>SNAMEETEAVQQDIEALEREIQTIKIQIANAHSGASKDEVKIPDAYKQFLSENINFSNLMRKDENTTLSINLSPRKPGTTTGQIQGIDSSIRSNFGVSSGHNEVAGFKSITDFVQWENSVRLIGVSLFPVNYDNIEFMGIRLELFDELSLKYDPPFYVILKPSVKRLGIWELFKHNLPKYINIHQHWQLITKDTDTSDSNIMKFANLCYKDLLKVHSRVQFFRKLEGNYVNDKQYSLLHIDNMGLNVSFRLGADIIKIKVDDGDDEIIDCTFNGEKNISLLGSIYGITNRFQSIIM[2x];>MDFTSSSGVLDSERNTGSNDSDEPSSHSDVIETEELKLIKLQEHKNNLLRQRSELLDQLSQTRVVEPRSVQLDDKLLLKLLRRNDNAVSDSSQSSNNPLPRVLPS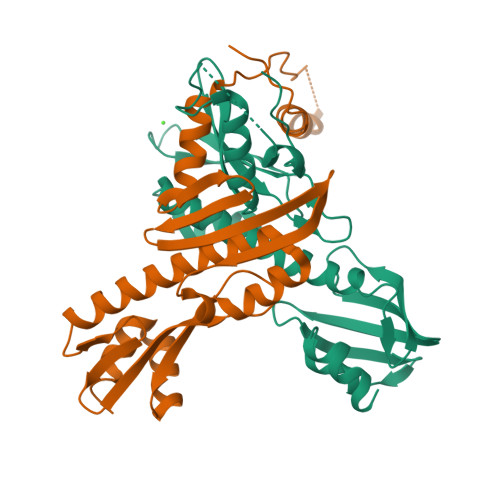LNIEQRKKYLDITLNDVTVTCEKDMILLRKGSFTASFRIAVENESIRSMAIDLNAFEVELQPIIQYAEDTQNVNVAMMAVVQFLRIKELHEQMISKIVEASKFIRASNNTITLNDLEVSFHCYWNLPSPYPETLILTNKVQKILDFLIYQYGIQLGVIKYGSTII[2x]The large terminase protein is a key component of the DNA packaging machinery in tailed bacteriophages and evolutionarily related herpes viruses. Typically, in addition to an ATPase domain which powers DNA translocation, the large terminase contains a nuclease domain which cuts concatemeric DNA, generated by rolling circle replication. Crystal structures of the large terminase nuclease from the thermophilic bacteriophage G20c show that it is most similar to the RuvC family of the RNase H-like endonucleases. The overall structure adopts the RNase-H fold.

Structures for complexes with Mn2+, Mg2+, Co2+ and Ca2+ were determined by soaking crystals of the apo protein, whereas the structure of the Zn2+ complex was obtained by co-crystallization. Only one metal ion, bound to the site A, was identified for conditions containing Mg2+, Mn2+ and Co2+. This metal ion is coordinated by the side chains of D294 and D429 and four water molecules in the canonical octahedral geometry. High resolution crystal structures of complexes with different metals reveal that in the absence of DNA, only one catalytic metal ion is accommodated in the active site. Like RuvC proteins, the nuclease requires either Mn2+, Mg2+ or Co2+ ions for activity, but is inactive with Zn2+ and Ca2+. Similar to G2P and UL89, addition of Mg2+ resulted only in limited activity, leading to production of nicked or linearized DNA when supercoiled DNA was used as substrate.

>GPAMNSVFSGLDMLILLPYERRGTRLVVEDYRPDHIYCIGADFGKNQDYSVFSVLDLDTGAIACLERMNGATWSDQVARLKALSEDYGHAYVVADTWGVGDAIAEELDAQGINYTPLPVKSSSVKEQLISNLALLMEKGQVAVPNDKTILDELRNFRYYRTASGNQVMRAYGRGHDDIVMSLALAYSQYEG[2x]5-amino-1-(pyridin-3-yl)-1H-imidazole-4-carboxamide | C9 H9 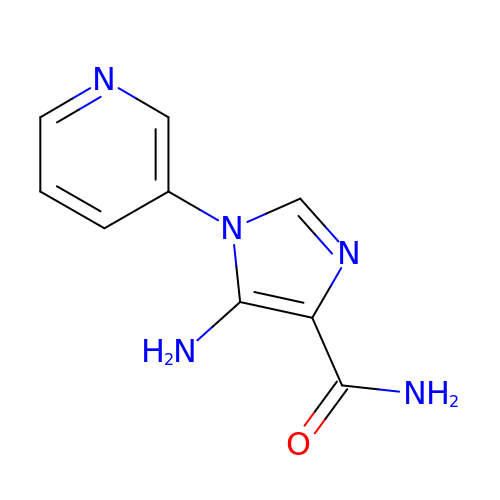N5 O | WZVCHXNAUQIDJM-UHFFFAOYSA-N>[2x]MCTSILYSPKDHYFGRNLDYEIAYGQKVVITPRNYEFKFANLPAEKSHYAMIGIAAVANNTPLYCDAINEKGLGVAGLSFAGQGKYFPVVEDKKNIASFEFISYILATYETVDQVKENLTDVNISDVSFSKNTPASELHWLVGDKTGKS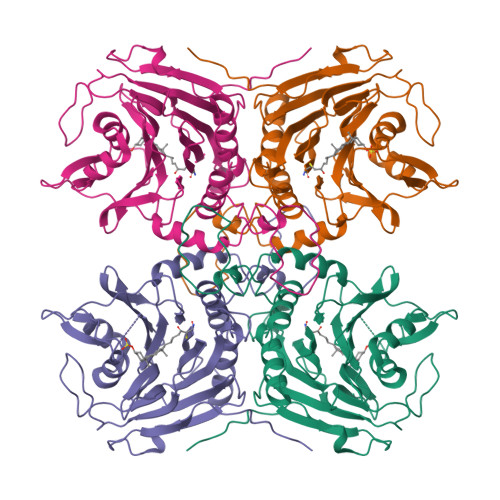IVVESDEKGLHVYDNPVNALTNAPLFPQQLTNLANYAAVVPGQPNNDFLPGVDLKMYSRSLGTHHLPGGMDSESRFVKVCFALNHAPKDSDEVESVTNFFHILQSVEQVKGMDEVGPNIFEYTMYTSCMNLEKGILYFNCYDDSRISAVDMNKEDLSSSDLIVFDLFKKQDISFINHHHHHH> GSHMSAEVIGQVEEALDTD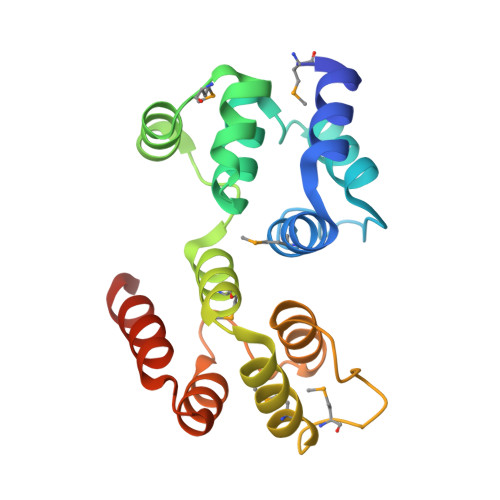EKEMLLFLCRDVAIDVVPPNVRDLLDILRERGKLSVGDLAELLYRVRRFDLLKRILKMDRKAVETHLLRNPHLVSDYRVLMAEIGEDLDKSDVSSLIFLMKDYMGRGKISKEKSFLDLVVELEKLNLVAPDQLDLLEKCLKNIHRIDLKTKIQKYKQSVQGAGTS>MKDNSTSAVSSWLGYKIQEYRLTQRLLEANNSSCIGFEILDDLEEHTGSTSTFEQDAISTTGRNIVSNHSKDLWKTLSNWMDLIDSGEIDVDNTIFLLFTNKRCHSEVLQLLSTSQATEEASKAFDEILKIVSHPSPSIANYLNNFSKSKTDACRLISKFTYIYGSGSAPHDLRESYKLHRLGALEEHLDEIMYEILGWVSDVLTLAAEKRQPTIVRAKDFGARLGEIESKYRQKTILNYFCNRSSESEDVQNTIKDAPNYIKQLNLINV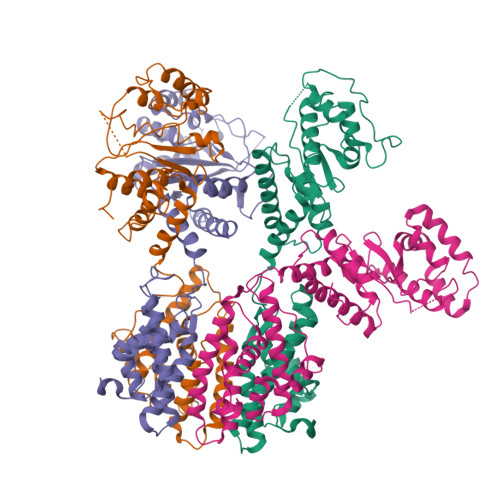DDSELEEAAIANLETKDAVVEWTLNGDVQDYSYRYYQRELRRCWGIQKQKIHLDFNGRPETEVGQRLYIECLNNVTRYYLENKKVGDFFAHGTLHSMADKLTIGWHPEFDKKLGDPDA[4x]>SELSFNYPNFQSVEDITFQGGASPRNETLQLTPTDSNGIPIRQRAGHAVYSQPFQLRDTSFYTTFTFVIRTTSNSPADGFAIFIAPPDFPVKRYGGYLGLFEPNTATNTSANKVVAVEFDTWVNTEWKE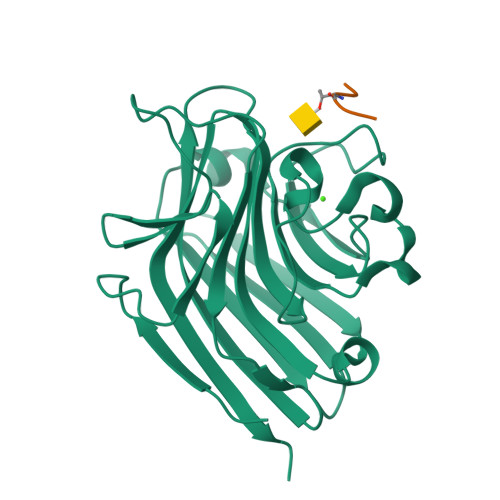PRYRHIGIDVNSIVSVRVTRWQDKDVFSRSIATAHVGYDGISKILTAFVTYPDGGNYVLSHVVDLAEIFPGDVRIGFSGATGQYETQYIHSWSFSSTSTNLLRDGARHHHHHH[10x];>XGVTSA[10x]Human SIDT1 and SIDT2 are closely related members of the SID-1 transmembrane family, and have been implicated in various biological processes such as glucose and lipid metabolism, innate immunity, and tumorigenesis. Here, we present the cryo-electron microscopy (cryo-EM) structures of human SIDT1 and SIDT2. Both structures reveal an overall architecture of a dimeric arrangement composed of an extracellular domain (ECD) rich in β-strands and a transmembrane domain (TMD) with 11 passes, highlighting the remarkable structural congruence. Importantly, the ECDs of SIDT1 and SIDT2 bind synthetic plant-derived miRNA only under acidic conditions.

SIDT2 also contains ten predicted N-glycosylation sites, with all six glycosylation sites on its ECD well resolved in the EM map, along with the corresponding disulfide bonds. A conserved hydrogen bond between S105 residues is observed in SIDT1, corresponding to S92 in SIDT2. In addition, Q113 in SIDT1 may maintain a hydrogen bond interaction with N219 from the other protomer instead of the ionic bond interaction observed between R100 and D204 in SIDT2. Furthermore, SIDT2 features an additional β-strand (residues 27–33) involved in interactions at the dimer interface, while the corresponding region in SIDT1 remains unstructured, indicating a high level of flexibility and fewer interactions at the dimer interface of SIDT1 compared to SIDT2. In the SIDT2 ECD model, the dimerization interaction involves a buried surface area of ~1700 Å2 from each protomer, in contrast to ~1300 Å2 in the SIDT1 model, indicating differences in the proximity of the formed homodimers between SIDT1 and SIDT2, probably due to sequence variations. Sedimentation velocity analytical ultracentrifugation (SV-AUC) analysis further confirmed that SIDT1ECD exists as a monomer, with a sedimentation coefficient of 2.8 S and a molecular weight of ~44.6 kDa, while SIDT2ECD forms a dimer with a sedimentation coefficient of 4.8 S and a molecular weight of ~74.2 kDa. The distinct ECD oligomerization states might be attributed to variations in amino acid composition and interactions at the dimer interface as shown in their structures. Furthermore, analysis of surface electrostatic potential on the ECD structures revealed positively charged regions on the β-strand surfaces of SIDT1 and SIDT2 ECDs at pH 7.5, with increased charge density and expanded distribution at pH 5.5. At pH 3.5, nearly all ECD regions displayed a positive charge, supporting the observed low-pH-dependent RNA-binding abilities of SIDT1 and SIDT2.

>[2x]MKANLLVLLCALAAADAHLGVLGPKNVSQKDAEFERTYVDEVNSELVNIYTFNHTVTRNRTEGVRVSVNVLNKQKGAPLLFVVRQKEAVVSFQVPLILRGMFQRKYLYQKVERTLCQPPTKNESEIQFFYVDVSTLSPVNTTYQLRVSRMDDFVLRTGEQFSFNTTAAQPQYFKYEFPEGVDSVIVKVTSNKAFPCSVISIQDVLCPVYDLDNNVAFIGMYQTMTKKAAITVQRKDFPSNSFYVVVVVKTEDQACGGSLPFYPFAEDEPVDQGHRQKTLSVLVSQA>[4x]SNAMKDKIIDNAITLFSEKGYDGTTLDDIAKSVNIKKASLYYHFDSKKSIYEQSVKCCFDYLNNIIMMNQNKSNYSIDALYQFLFEFIFDIEERYIRMYVQLSNTPEEF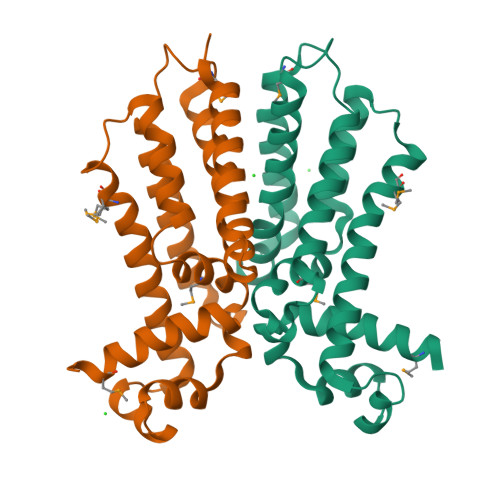SGNIYGQIQDLNQSLSKEIAKFYDESKIKMTKEDFQNLILLFLESWYLKASFSQKFGAVEESKSQFKDEVYSLLNIFLKK>MASVNPEYFSAADVYVPDEWEVAREKITMSRELGQGSFGMVYE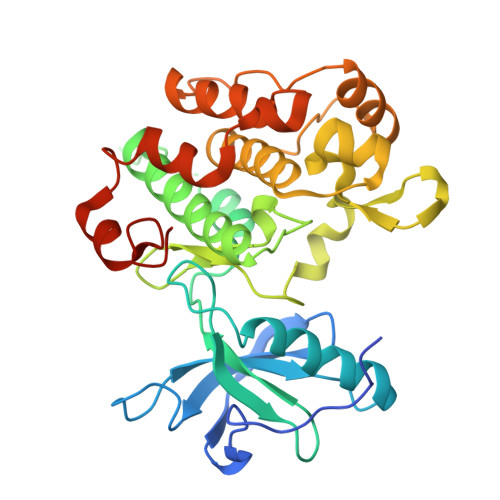GVAKGVVKDEPETRVAIKTVNEAASMRERIEFLNEASVMKEFNCHHVVRLLGVVSQGQPTLVIMELMTRGDLKSYLRSLRPEMENNPVLAPPSLSKMIQMAGEIADGMAYLNANKFVHRDLAARNCMVAEDFTVKIGDFGMTRDIYETDYYRKGGKGLLPVRWMSPESLKDGVFTTYSDVWSFGVVLWEIATLAEQPYQGLSNEQVLRFVMEGGLLDKPDNCPDMLFELMRMCWQYNPKMRPSFLEIISSIKEEMEPGFREVSFYYSEENKLPEPEELD[2x]>GHMAKRVFFSFHYQDVIDFRVNVVRNHWVTKLNQSAAGVFDASLWEDAKKTSDIALKRLINGGLNNTSVTCVLIGSQTFNRRWVRYEIMKSIEKGNKIIGIHINAFKDKYGNIKSKGPNPFDYLGYQYSSDGKQLHLYEWTGGKWEEYKDLAPYRVNQIAPESLRGKFYSLSSVYRVYDWVADDGYNKFSSWVN[2x]

The Thoeris system is composed of two genes, thsA and thsB. In the present study, we report structural and functional analyses of the ThsA and ThsB proteins from the B. cereus Thoeris defense system. Crystal structures of ThsA and ThsB were determined to resolutions of 2.5 and 1.8 Å, respectively. Combined with previous findings, these results advance our understanding of the molecular mechanism underlying the Thoeris defense system and suggest that NAD+ degradation is a previously unknown strategy for bacterial antiphage resistance.

To gain structural insight into the role of ThsB in the Thoeris defense system, we determined the crystal structure of B. cereus ThsB. Two ThsB molecules were found in the asymmetric unit, and the RMSD value of the Cα atoms was only 0.9 Å, indicating high similarity. ThsB exhibited a four-layered structure in which α-helices and β-sheets were alternately stacked. A five-stranded parallel β-sheet (β2–β1–β3–β4–β10) and five α-helices comprise the Rossmann-like fold, with α1, α2, and α5 on the concave side of the β-sheet and α3 and α4 on the convex side. An additional antiparallel β-sheet (β5–β9) is located adjacent to the α4 helix in an approximately parallel orientation. However, excluding the additional antiparallel β-sheet, the Rossmann-like fold portion of ThsB revealed a structural resemblance to TIR domain proteins such as human sterile alpha and TIR motif containing 1 (SARM1), nucleoside monophosphate hydrolases, and toll-like receptors. Despite the high structural similarity to SARM1, ThsB did not cleave NAD+ in our in vitro assay. By contrast, our SEC-MALS analysis indicated that ThsB exists as a monomer even at high concentrations (~1 mM). When expressing (His)6-maltose binding protein (MBP)-tagged ThsA together with untagged ThsB in E. coli cells, ThsB did not co-purify with ThsA in nickel-affinity chromatography. These observations suggest that ThsB does not form a stable complex with ThsA. On this basis, we tested the hydrolase activity of ThsB in the presence of various ribonucleotides such as AMP, GMP, UMP, and CMP, but no hydrolysis was detected. This raises other possibilities; the enzymatic activity of ThsB may be triggered by an unknown in vivo mechanism, or ThsB may have nonenzymatic function(s) as a toll-like receptor.> MNKAKRLEILTRLRENN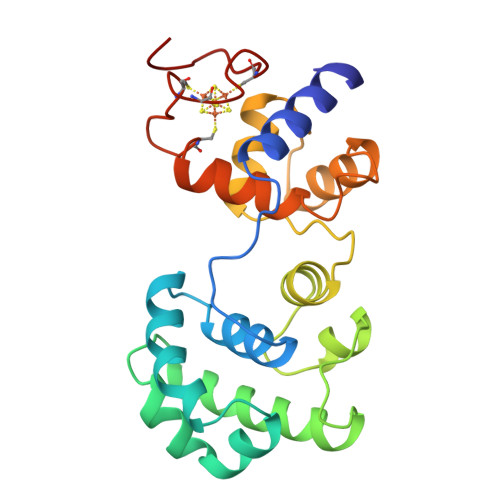PHPTTELNFSSPFELLIAVLLSAQATDVSVNKATAKLYPVANTPAAMLELGVEGVKTYIKTIGLYNSKAENIIKTCRILLEQHNGEVPEDRAALEALPGVGRKTANVVLNTAFGWPTIAVDTHIFRVCNRTQFAPGKNVEQVEEKLLKVVPAEFKVDCHHWLILHGRYTCIARKPRCGSCIIEDLCEYKEKVDI> SQDFITIGTGSVTGVYYPTGGAICKLVNKDRKDHNIRCSVESTGGSIYNVNTIRSGELD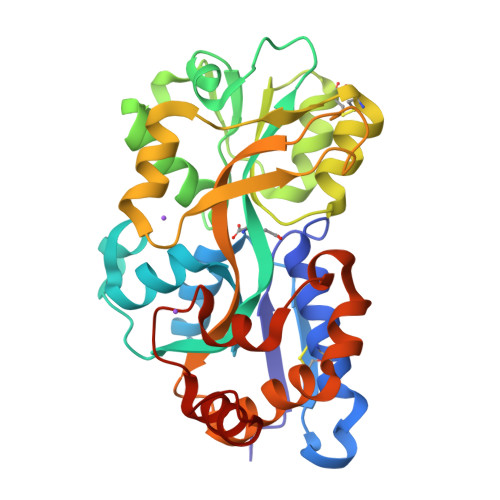FGIVQSDWQYHGYNGTSEFAEQGPYKKLRAVFSMHTEPFNIIARADSGIENVKDLAGKRVNIGNPGSGDRATMQVVMDAFGWNNDSFKLAAELKGSERSQALCDNKIDAFIYMVGHPNGAIKEATTSCAAKLVPATGPEIEKIVANNPYYAYSVVPAGMYSGTDQEVKSFGVAATLVTTEEVSEAVVYNLTKAVFENFDTFTRLHPAFANLKKEDMVTAGNSIPLHPGAVKYYKEAGLIK>GSTWRQNTKSSRIEAIKIQILSKLRLETAPNISKDVIRQLLPKAPPLRELIDQYDVQRDDSSDGSLEDDDYHATTETIITMPTESDFLMQVDGKPKCCFFKFSSKIQYNKVVKAQLWIYLRPVETPTTVFVQILRLIKPMKDGTRYTGIRSLKLDMNPGTGIWQSIDVKTVLQNWLAAPASNLGIEIKALDENGHDLAVTFPGPGEDGLNPFLEVKVTDTPKRSRRDFG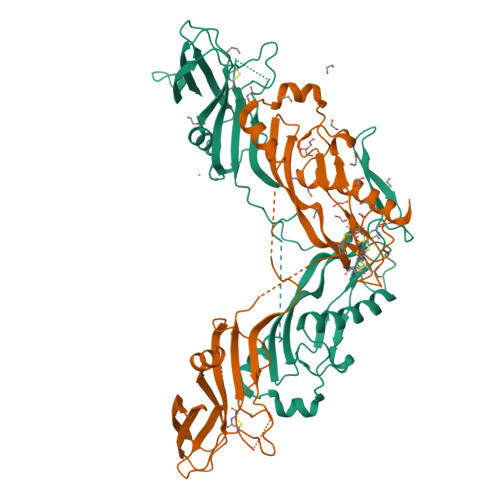LDCDEHSTESRCCRYPLTVDFEAFGWDWIIAPKRYKANYCSGECEFVFLAAYPHTHLVHQANPRGSAGPCCTPTKMSPINMLYFNGKEQIIYGKIPAMVVDRCGCS[2x]> MSLKKIQFFDTTLRDGEQTPGVNFDVKEKIQIALQLEKLGIDVIEAGFPISSPGDFECVKAIAKAIKHCSVTGLARCVEGDIDRAEEALKDAVSPQIHIFLATSDVHMEYKLKMSRAEVLASIK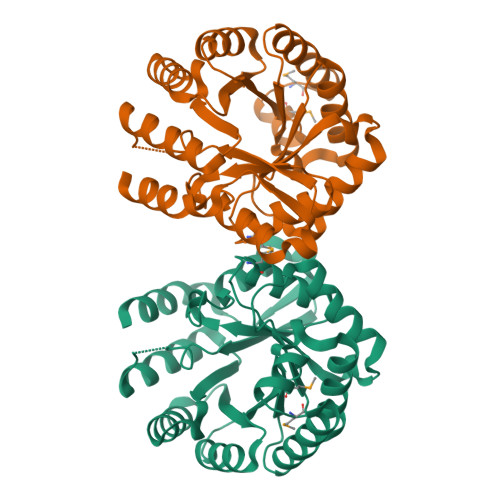HHISYARQKFDVVQFSPEDATRSDRAFLIEAVQTAIDAGATVINIPDTVGYTNPTEFGQLFQDLRREIKQFDDIIFASHCHDDLGMATANALAAIENGARRVEGTINGIGERAGNTALEEVAVALHIRKDFYQAETNIVLNQFKNSSDLISRLSGMPVPRNEGHHHHHH(7R)-2-[(3,5-difluoro-4-hydroxyphenyl)amino]-5,7-dimethyl-8-(3-methylbutyl)-7,8-dihydropteridin-6(5H)-one 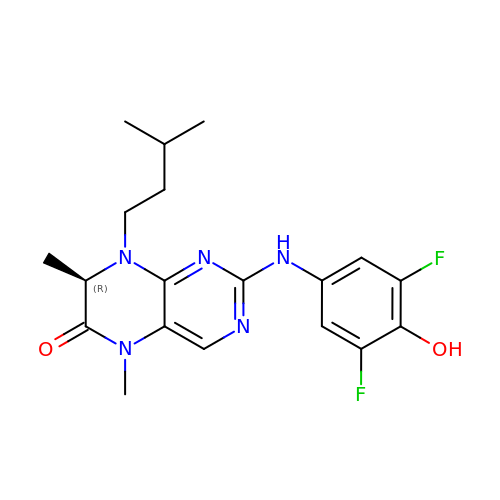| C19 H23 F2 N5 O2 | DTEKTGDVSARYDS-LLVKDONJSA-N>[2x]MEPSDQKVDTVPQYLKQSHERIFENNRA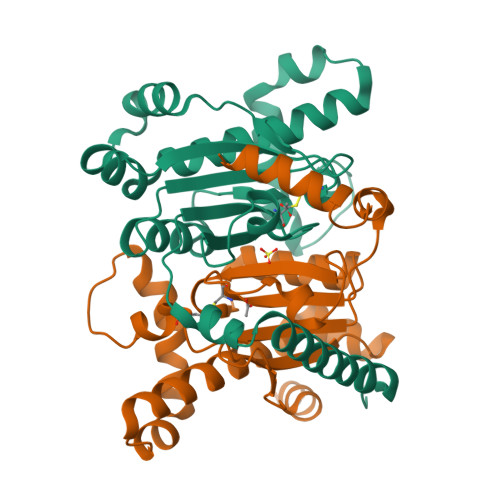WVATKMKDDPAFFEKLSAGQTPEYLYIGCSDSRVPANEIMGLEAGEVFVHRNIANLVPNTDLNVMSVINYAVRHLQVKHIVVCGHYHCGGVKAALTPSDLGLLNPWLRNVRDVYRLHEQELDGIQDATARYRRLVELNVIESCRNVIKTAAVQQSFHERQFPVVHGWIFDVETGLLRDLEIDFEETLRDIKKIYNLAPGS4-chloranyl-2-methyl-5-[(2-methyl-3,4-dihydro-1~{H}-isoquinolin-5-yl)amino]pyridazin-3-one | 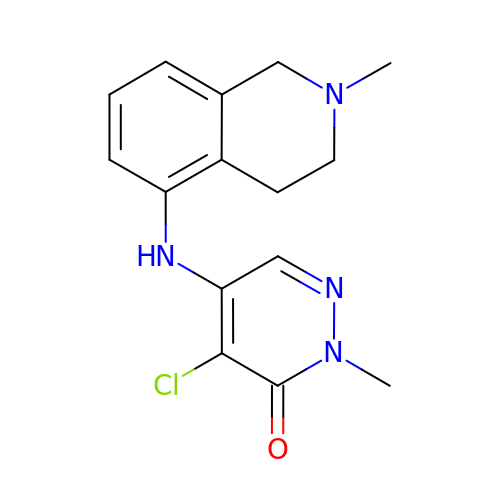C15 H17 Cl N4 O | YJJYUKCKKSVTAG-UHFFFAOYSA-N As the virus buds from the cell, the viral protease cleaves Gag into several fragments, including the capsid protein (CA) that then assembles into the mature capsid shell (core), rendering the virus particle infectious. The CA portion of all retroviral Gag proteins folds into two separate domains, the N-terminal domain (CANTD) and C-terminal domain (CACTD). In mature lattices, CANTD interactions form only intra-hexamer and intra-pentamer interfaces, while CACTD interactions are also involved in formation of inter-hexamer and inter-pentamer interfaces. Our results show that, like lentiviruses, RSV is sensitive to IP6 in vitro and in cells, where in the mature CA lattice IP6 binds in a pore formed in the center of the CANTD hexamer.

High concentrations of NaPO4 are known to induce RSV CA to assemble predominantly into T = 1 icosahedral CLPs, which consist of only 12 pentamers. The observation that within pleomorphic polyhedrons the CA pentamer constitutes the rigid building block prompted us to investigate if the pentamers within T = 1 icosahedrons and polyhedrons are structurally identical. Hence, we acquired cryo-EM micrographs of T = 1 icosahedral CLPs and subjected them to single-particle analysis, yielding a 3.1 Å resolution reconstruction. At this resolution refinement of RSV CA into the EM density was unambiguously possible. We compared the model of T = 1 pentamers with the model of the pentamer derived from the polyhedrons. In fact, the two models are virtually superimposable, showing an RMSD of their C-alpha atoms of 0.74 Å. This finding further underscores the observations that the RSV CA pentamer (1) is very rigid due to the tighter packing of the CA domains in the pentamer, (2) always promotes the same local geometry, and (3) is independent in arrangement of the size and shape of the CLP. In contrast, the increased flexibility of the RSV hexamer allows a more random distribution of pentamers in mature RSV cores. This enables RSV CA to even form inter-pentameric contacts, which can be regularly observed on polyhedrons and in particular T = 1 icosahedral particles.

> PVVIKTEGPAWTPLEPKLITRLADTVRTKGLRSPITMAEVEALMSSPLLPHDVTNLMRVILGPAPYALWMDAWGVQLQTVIAAATRDPRHPANGQGRGERTNLNRLKGLADGMVGNPQGQAALLRPGELVAITASALQAFREVARLAEPAGPWADIMQGPSESFVDFANRLIKAVEGSDLPPSARAPVIIDCFRQKSQPDIQQLIRTAPSTLTTPGEIIKYVLDRQKTA> MAAPVVAPPGVVVSRANKRSGAGPGGSGGGGARGAEEEPPPPLQAVLVADSFDRRFFPISKDQPRVLLPLANVALIDYTLEFLTATGVQETFVFCCWKAAQIKEHLLKSKWCRPTSLNVVRIITSELYRSLGDVLRDVDAKALVRSDFLLVYGDVISNINITRALEEHRLRRKLEKNVSVMTMIFKESSPSHPTRCHEDNVVVAVDSTTNRVLHFQKTQGLRRFAFPLSLFQGSSDGVEVRYDLLDCHISICSPQVAQLFTDNFDYQTRDDFVRGLLVNEEILGNQIHMHVTAKEYGARVSNLHMYSAVCADVIRRWVYPLTPEANFTDSTTQSCTHSRHNIYRGPEVSLGHGSILEENVLLGSGTVI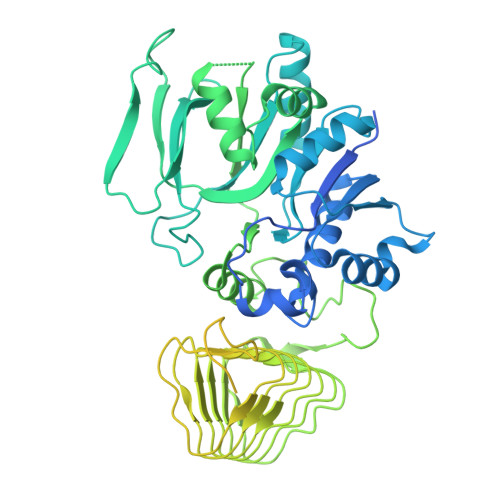GSNCFITNSVIGPGCHIGDNVVLDQTYLWQGVRVAAGAQIHQSLLCDNAEVKERVTLKPRSVLTSQVVVGPNITLPEGSVISLHPPDAEEDEDDGEFSDDSGADQEKDKVKMKGYNPAEVGAAGKGYLWKAAGMNMEEEEELQQNLWGLKINMEEESESESEQSMDSEEPDSRGGSPQMDDIKVFQNEVLGTLQRGKEENISCDNLVLEINSLKYAYNISLKEVMQVLSHVVLEFPLQQMDSPLDSSRYCALLLPLLKAWSPVFRNYIKRAADHLEALAAIEDFFLEHEALGISMAKVLMAFYQLEILAEETILSWFSQRDTTDKGQQLRKNQQLQRFIQWLKEAEEESSEDD(2S)-2-({(2S)-3-[(R)-[(1R)-1-({(4S)-4-amino-5-[(2S)-2-cyanopyrrolidin-1-yl]-5-oxopentanoyl}amino)ethyl](hydroxy)phosphoryl]-2-benzylpropanoyl}amino)propanoic 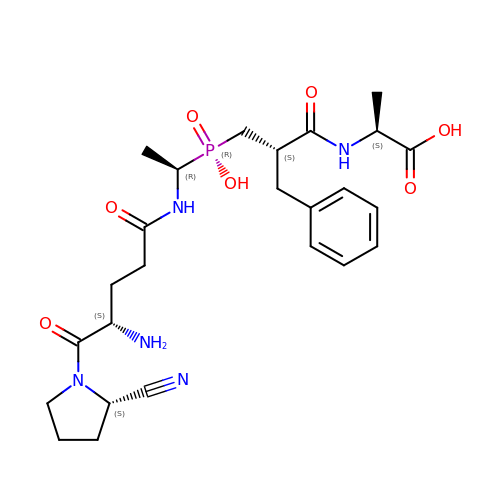acid | C25 H36 N5 O7 P | BNNCRIIZOMKDCO-TYIUSFPZSA-N3-methoxybenzyl 3-methyl-4-(piperidin-4-yloxy)-1-benzofuran-2-carboxylate | C23 H25 N O5 | 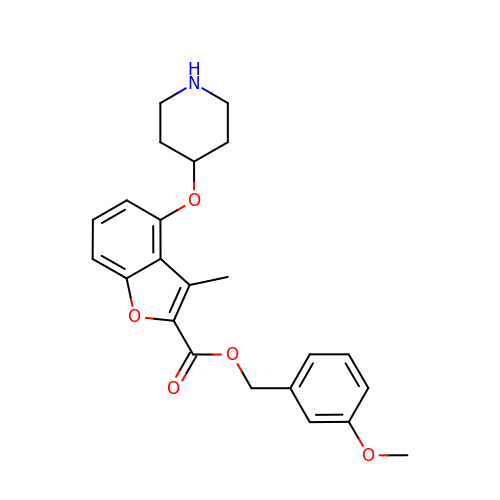MODWRRKHFAUNLX-UHFFFAOYSA-N>MAQSKGSVDQTLHAPHCEVGCAANVARRVGVDLARQVIGAHWASRMLVREVGTFPQPLLDRTQVTFSAQGEGWPALLARMTGGEVTSRHVPREELLSTLHADRAEGGTLLFMEDRACPWLDSAHSPGMLPHVVVPDGVAPDGSWQLIEGHSWWRGRYAMSEQDLLAASYPDPDPHHVAGRVLSLRIRPSAERAAQLDTLARQELAAGLRTYLAAECGETETPAGRIVWANGPQSVPLLVERLRGWDYLCPLAARNDLSTEHARDVALGRYLFLALTDEL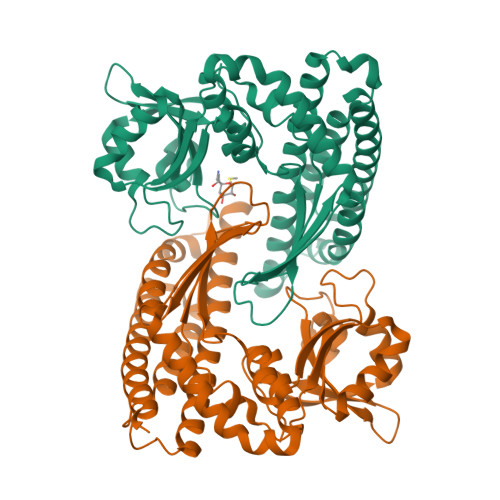AFAAYARAGTLRLVEGLGLAGAVGGLRPDEAWRLAWRSGQKLYRRLDRQNLSALFSALEKAAEVDVEYARRLLKELLEHHHHHHHH[2x]>MIVKKLTLPKDFLWGGAVAAHQVEGGWNKGGKGPSICDVLTGGAHGVPREITKEVLPGKYYPNHEAVDFYGHYKEDIKLFAEMGFKCFRTSIAWTRIFPKGDEAQPNEEGLKFYDDMFDELLKYNIEPVITLSHFEMPLHLVQQYGSWTNRKVVDFFVRFAEVVFERYKHKVKYWMTFNEINNQRNWRAPLFGYCCSGVVYTEHENPEETMYQVLHHQFVASALAVKAARRINPEMKVGCMLAMVPLYPYSCNPDDVMFAQESMRERYVFTDVQLRGYYPSYVLNEWERRGFNIKMEDGDLDVLREGTCDYLGFSYYMTNAVKAEGGTGDAISGFEGSVPNPYVKASDWGWQIDPVGLRYALCELYERYQRPLFIVENGFGAYDKVEEDGSINDDYRIDYLRAHIEEMKKAVTY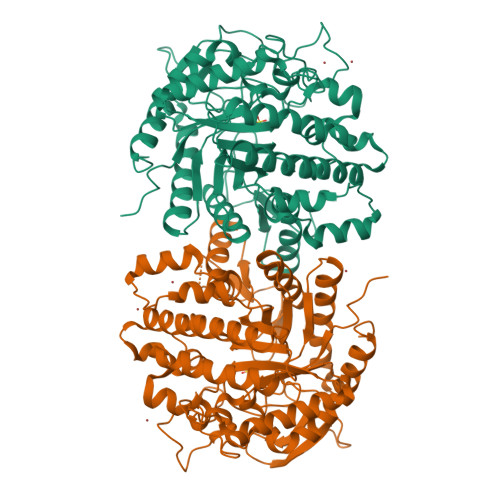DGVDLMGYTPWGCIDCVSFTTGQYSKRYGFIYVNKHDDGTGDMSRSRKKSFNWYKEVIASNGEKL[4x]>[4x]KKSWDEMSCAEKLFKVLSFGLWNPTYSRSERQSFQELLTVLEPVYPLPNELGRVSARFSDGSSLRISVTNSELVEAEIRTANNEKITVLLESNEQNRLLQSLPIDRHMPYIQVHRALSEMDLTDTTSMRNLLGFTSKLSTTLIPHNAQTDPLSGPTPFSSIFMDTCRGLGNAKLSLNGVDIPANAQKLLRDALGLKDTHSSPTRNVIDHGISRHDAEQIARESSGSDKQKAEVVEFL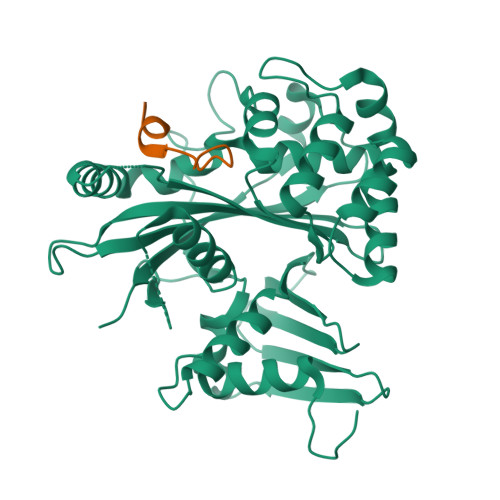CHPEAATAICSAFYQSFNVPALTLTHERISKASEYNAERSLDTPNACINISISQSSDGNIYVTSHTGVLIMAPEDRPNEMGMLTNRTSYEVPQGVKCIIDEMVSALQPRYAASETYLQNT;>QAVLDVLKFYDSNTVK[4x]> TTIVALKYPGGVVMAGDRRSTQGNMISGRDVRKVYITDDYTATGIAGTAAVAVEFARLYAVELEHYEKLEGVPLTFAGKINRLAIMVRGNLAAAMQGLLALPLLAGYDIHASDPQSAGRIVSFDAAGGWNIEEEGYQAVGSG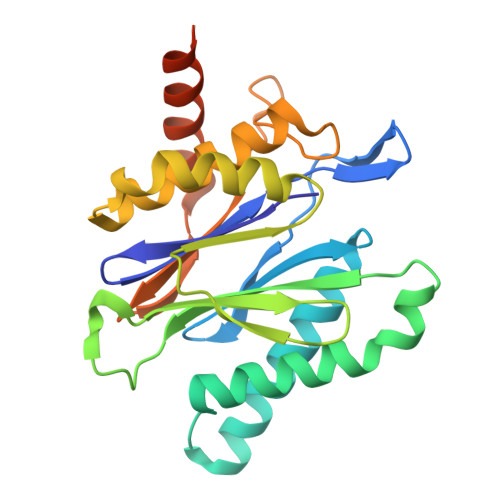SLFAKSSMKKLYSQVTDGDSGLRVAVEALYDAADDDSATGGPDLVRGIFPTAVIIDADGAVDVPESRIAELARAIIESRSGADTFGSDGGEKHHHHHH> TTQLIQQVSLTDFFRPDIEHAGSTVLILRHPTDLPHLARHRAPPGRQTERLAE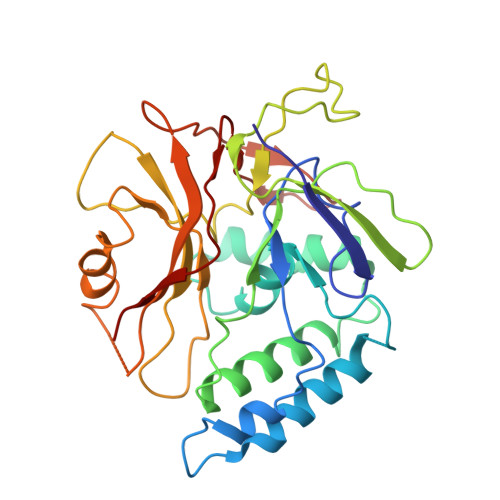AWGQLLEASESGCARAYVTSLSFIAACRAEEYTDKQAAEANRTAIVSAYGCSRMGARLIRFSECLRAMVQCHVFPHRFISFFGSLLEYTIQDNLCNITAVAKGPQEAARTDKTSTRRVTANIPACVFWDVDKDLHLSADGLKHVFLVFVYTQRRQREGVRLHLALSQLNEQCFGRGIGFLLGARICMYAAYTLIGTIPSESVRYTRRMERFGGYNVPTIWLEGVVWGGTNTWNECY> GSSTNIDKVNLFILGKDGLAQELANEIRTQSTDDEYALDGKIYELDLRPVDAKSPYFLSQLWTAAFKPHGCFCVFNSIESLSFIGEFIGKIRTEASQIRKDKYMANLPFTLILANQRDSISKNLPILRHQGQQLANKLQCPFVDVPAGTYP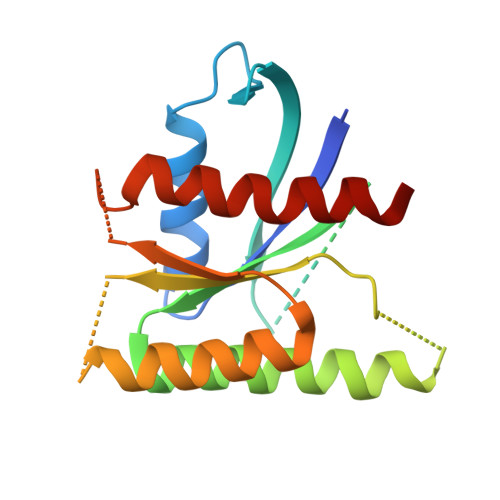RKFNETQIKQALRGVLESVKHNLDV Nylon hydrolase (NylC) is one of the three enzymes responsible for the endo-type degradation of the by-products of nylon-6 manufacture (cyclic and linear oligomers of 6-aminohexanoate (Ahx) with a degree of polymerization greater than three) and various aliphatic nylons (e.g., nylon-6 and nylon-66). However, the post-translational autocleavage of the nascent polypeptide between Asn266 and Thr267 generates an active enzyme with an α subunit (27 kDa) and a β subunit (9 kDa). Based on the X-ray-crystallographic structure of NylCA, we reported that four αβ heterodimers (molecules A-D) form a doughnut-shaped quaternary structure. In addition, we proposed that the nucleophilic N-terminal residue Thr267 in the β subunit functions as a catalytic residue for either autocleavage (from precursor to active enzyme) or substrate hydrolysis.

His130 and Leu137 in NylCp2 were located in a loop between helix α1 and β-strand β7 (designated “loop 3”). Three amino acid residues corresponding to the substitutions D122G, H130Y, and D36A (increasing the protein stability of NylCp2) and one amino acid residue corresponding to the substitution L137A (decreasing the protein stability) were located at the A/D interface, and the glutamate residue corresponding to the substitution E263Q was found at the A/B interface.

>[2x]MNTTPVHALTDIDGGIAVDPAPRLAGPPVFGGPGNDAFDLAPVRSTGREMLRFDFPGVSIGAAHYEEGPTGATVIHIPAGARTAVDARGGAVGLSGGYDFNHAICLAGGAGYGLEAGAGVSDALLERLEYRTGFAELQLVSSAVIYDFSARSTAVYPDKALGRAALEFAVPGEFPQGRAGAGMSASAGKVDWDRTEITGQGAAFRRLGDVRILAVVVPNPVGVIVDRAGTVVRGNYDAQTGVRRHPVFDYQEAFAEQVPPVTEAGNTTISAIVTNVRMSPVELNQFAKQVHSSMHRGIQPFHTDMDGDTLFAVTTDEIDLPTTPGSSRGRLSVNATALGAIASEVMWDAVLEAGK>[2x]MGSSHHHHHHSSGRENLYFQGHMTNLVDKAAHSFATQNVVFQTLATASGKLVGVVTLNVEKALNALDLDMVRAMTVQLNLWKKDPLIACVVLDGSGEKAFCAGGDVRALYHASVAAKGQVTEVAKVFFEEEYRLDYLLHTYGKPVLVWGDGIVMGGGLGLMAGASHKVVTETSRIAMPEVTIGLYPDV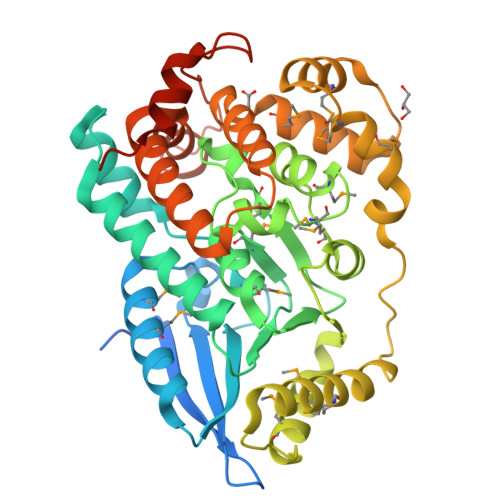GGSYFLNRMPGKMGLFLGLTAYHMNAADACYVGLADHYLNRDDKELMFDAMATLDWSDSPALNHQRLDTMINELSNQVDIPKGDSVLAESQEMIDRLMAGSLTDIVTRMSTLSTDEAWLSKACATMLAGSPISWHLAYIQTQLGTKLSLAQCFKWELTVSVNVCAKGDFCEGVRALLIDKDKQPKWQFADVQSVPNSVIEDILTSPWGEEHPLSQLSGS>[2x]MSSQKVFGITGPVSTVGATAAENKLNDSLIQELKKEGSFETEQETANRVQVLKILQELAQRFVYEVSKKKNMSDGMARDAGGKIFTYGSYRLGVHGPGSDID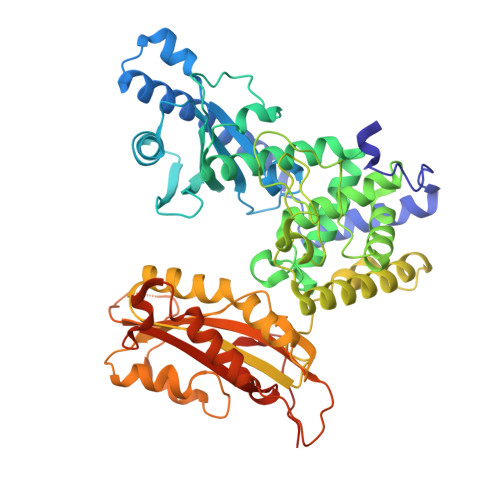TLVVVPKHVTREDFFTVFDSLLRERKELDEIAPVPDAFVPIIKIKFSGISIDLICARLDQPQVPLSLTLSDKNLLRNLDEKDLRALNGTRVTDEILELVPKPNVFRIALRAIKLWAQRRAVYANIFGFPGGVAWAMLVARICQLYPNACSAVILNRFFIILSEWNWPQPVILKPIEDGPLQVRVWNPKIYAQDRSHRMPVITPAYPSMCATHNITESTKKVILQEFVRGVQITNDIFSNKKSWANLFEKNDFFFRYKFYLEITAYTRGSDEQHLKWSGLVESKVRLLVMKLEVLAGIKIAHPFTKPFESSYCCPTEDDYEMIQDKYGSHKTETALNALKLVTDENKEEESIKDAPKAYLSTMYIGLDFNIENKKEKVDIHIPCTEFVNLCRSFNEDYGDHKVFNLALRFVKGYDLPDEVFDENEKRPSKKSKRKNLLEHHHHHH> MAAAPQINAELVTANLEAFLELMPEMGERLRVHRPQSNLVVNEDGDLDVEFRGEFLYGPGGRKRIEDMATRTALGPDHRISAAPLSSGHVDLIVKRFLYNILKRATDSGLSFLQHPEESGGFHMVCLGLGLGYQLPILLEQDNPAGIHIVEPNFDFLYHSLSTVDWRPLLETRRENPLRLNIIIEEEPGQIARQLRSAIRCCCPIVVDWTRLFVAYNSPLLTAAMSEFMRDAQLIGIGLGFLHDEMEMTRASYKNMRDGRYSILQHSATQLHTPVFIVGSGPSIDDDIEVIKANQDRAVIISCGTASRVLLANGIQPDFQMLLENGAAPYRALAAVHEEFGFGSA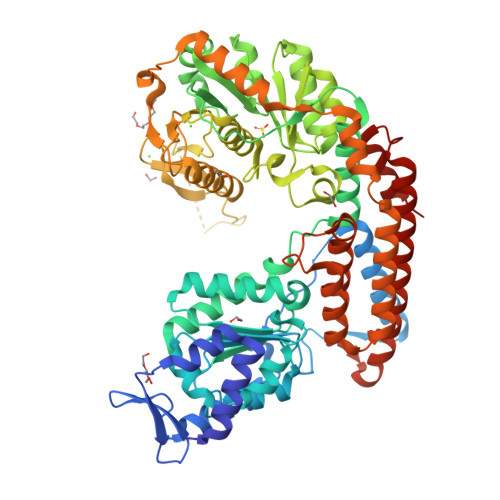TLIGSNTVDPRVRDLFEDVVYYFRPALSSYALFSPGIEYSLDDSGPTVTNTGTTAALALGFRELYLFGVDLGSRNPKRHHSKQSLYRHADDTKDGQKGAMDFDAVFDVREPGNFGGVVYSETIMLWTRDALGRIIGRYRPAANAFNCSDGVMIENTRPLSSQSLRLKSTPDMKAKDLAKVRASFRPGGEELFHDRWDREDWPRSIVTLLGECAQAMDDHVGDSNRLMLVLSEMLLRDYKQPPTVAQFFVRGTLMMAAMCYDYYVKRVTPADRKAEFWEIIRDEFHQMIRVMTLQVEWYFDNIEAFESDEELFDKVTGWDYD> MGSSHHHHHHMVMLHSKNVKGFLENTLKPYDLHSVDFKTSSLQSSMIITATNGGILSYATSNNDVPKNSINEINSVNNLKMMSLLIKDKWSEDENDTEEQHSNSCYPVEIDSFKTKIYTYEMEDLHTCVAQIPNSDLL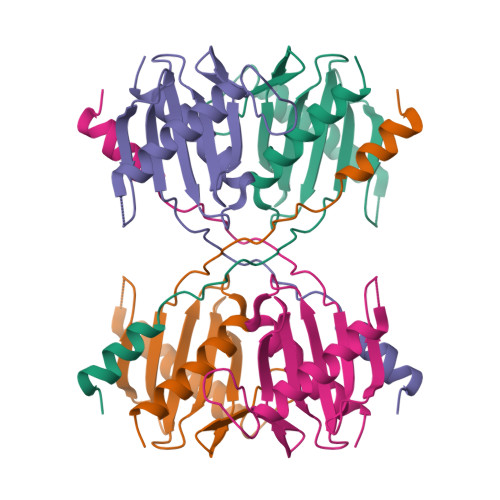LLFIAEGSFPYGLLVIKIERAMRELTDLFGYKLG> GPLGSMEASCLELALEGERLCKSGDCRAGVSFFEAAVQVGTEDLKTLSAIYSQLGNAYFYLHDYAKALEYHHHDLTLARTIGDQLGEAKASGNLGNTL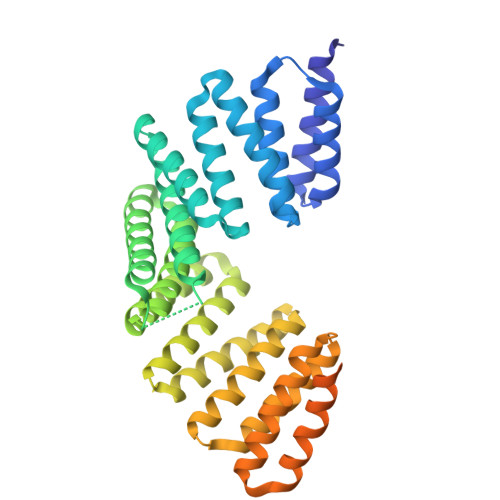KVLGNFDEAIVCCQRHLDISRELNDKVGEARALYNLGNVYHAKGKSFGCPGPQDVGEFPEEVRDALQAAVDFYEENLSLVTALGDRAAQGRAFGNLGNTHYLLGNFRDAVIAHEQRLLIAKEFGDKAAERRAYSNLGNAYIFLGEFETASEYYKKTLLLARQLKDRAVEAQSCYSLGNTYTLLQDYEKAIDYHLKHLAIAQELNDRIGEGRACWSLGNAYTALGNHDQAMHFAEKHLEISREVGDKSGELTARLNLSDLQMVLGLSYSTNNSIMSENTEIDSSLNGVRPKLGRRHSMENMELMKLTPEK> NQQICDRYGTTTIQDRYVVQNNRWGTSATQCINVTGNGFEITQADGSVPTNGAPKSYPSVYDGCHYGNCAPRTTLPMRISSIGSAPSSVSYRYTGNGVYNAAYDIWLDPTPRTNGVNRTEIMIWFNRV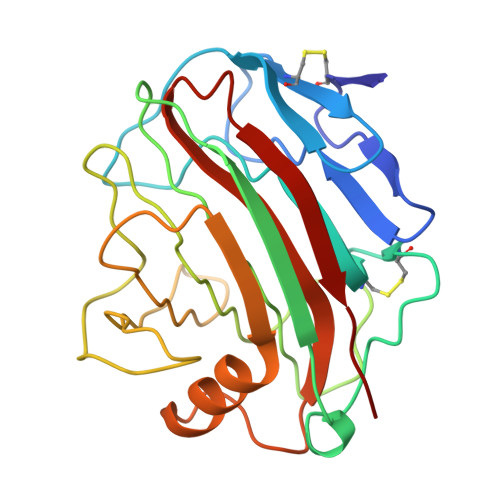GPVQPIGSPVGTAHVGGRSWEVWTGSNGSNDVISFLAPSAISSWSFDVKDFVDQAVSHGLATPDWYLTSIQAGFEPWEGGTGLAVNSFSSAVNA>[2x]GSAMAKANSSFSEVQI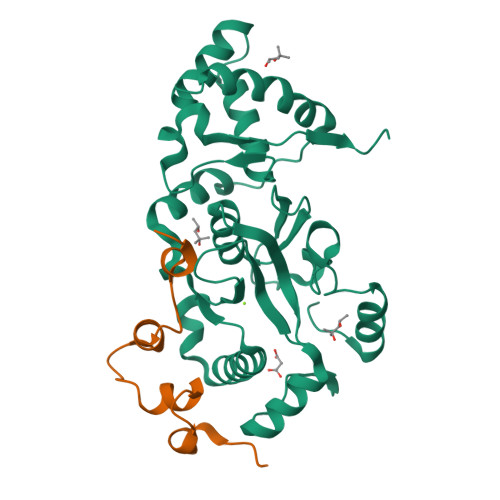ARRIKEGRGQGHGKDYIPWLTVQEVPSSGRSHRIYSHKTGRVHHLLSDLELAVFLSLEWESSVLDIREQFPLLPSDTRQIAIDSGIKHPVIRGVDQVMSTDFLVDCKDGPFEQFAIQVKPAAALQDERTLEKLELERRYWQQKQIPWFIFTDKEINPVVKENIEWLYSVKTEEVSAELLAQLSPLAHILQEKGDENIINVCKQVDIAYDLELGKTLSEIRALTANGFIKFNIYKSFRANKCADLCISQVVNMEELRYVAN;>[2x]GSAIKVVKPSDWDSLPDTDLRYIYSQRQPEKTMHERLKGKGVIVDMASLFKQAG> IHDFCLVSKVVGRCRASMPRWWYNV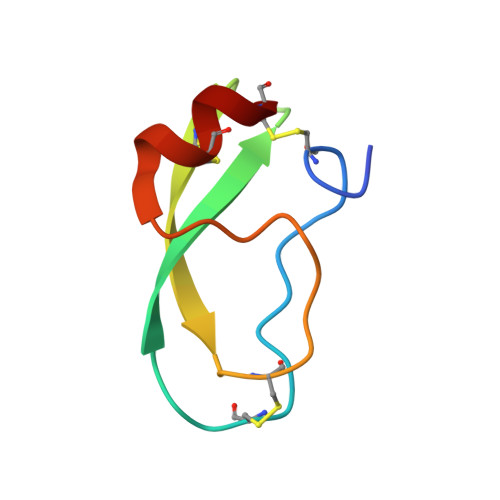TDGSCQLFVYGGCDGNSNNYLTKEECLKKC>[6x]SAAQKFVKQVIREAFLQDASDIHIEPRQN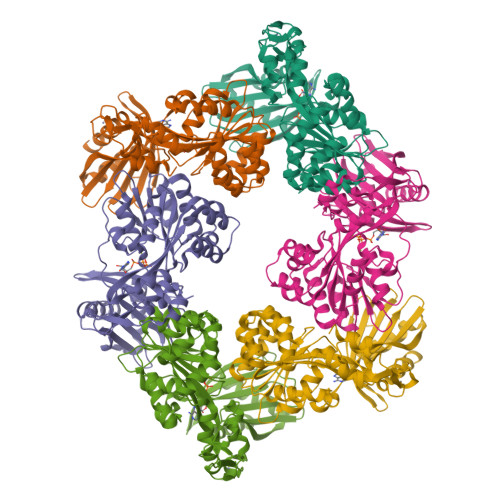DVQVRLRIDGALRPYSTLPKGALNAVISVVKIMGGLNIAEKRLPQDGRVRYREGAIDVDLRLSTLPTVYGEKAVMRLLKKASDIPEIEDLGFAPGVFERFKEVISKPYGIFLITGPTGSGKSFTTFSILKRIATPDKNTQTIEDPVEYEIPGINQTQVNPQAGLTFARALRAFLRQDPDIIMVGEIRDSETAKIATEAALTGHLVIATLHTNDAAQAITRLDEMGVEPFNISAALIGVLSQRLVRRVCEHCKVEVKPDPETLRRLGLSEAEIQGARLYKGMGCERCGGTGYKGRYAIHELLVVDDEIRHAIVAGKSATEIKEIARRKGMKTLREDGLYKALQGITTLEEVLARTIE> MGSDKIHHHHHHMKEIDELTIKEYGVDSRILMERAGISVVLAMEEELGNLSDYRFLVLCGGGNNGGDGFVVARNLLGVVKDVLVVFLGKKKTPDCEYNYGLYKKFGGKVVEQFEPSILNEFDVVVDAIFGTGLRGEITGEYAEIINLVNKSGKVVVSVDVPSGIDSNTGKVLRTAVKADLTVTFGVPKIGHILFPGRDLTGKLKVANIGHPVHLINSINRYVITREMVRSLLPERPRDSHKGTYG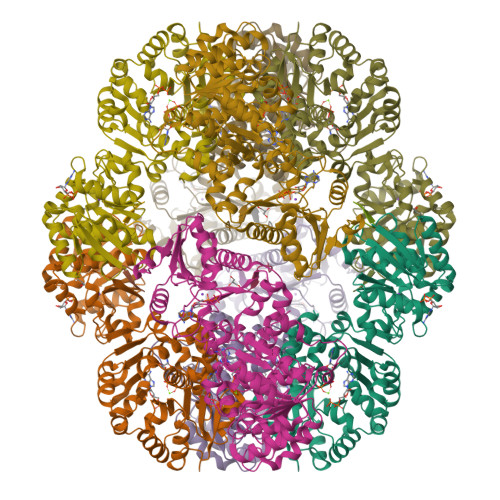KVLIIAGSRLYSGAPVLSGMGSLKVGTGLVKLAVPFPQNLIATSRFPELISVPIDTEKGFFSLQNLQECLELSKDVDVVAIGPGLGNNEHVREFVNEFLKTLEKPAVIDADAINVLDTSVLKERKSPAVLTPHPGEMARLVKKTVGDVKYNYELAEEFAKENDCVLVLKSATTIVTDGEKTLFNITGNTGLSKGGSGDVLTGMIAGFIAQGLSPLEASTVSVYLHGFAAELFEQDERGLTASELLRLIPEAIRRLKE;> AAWLFEA ethyl 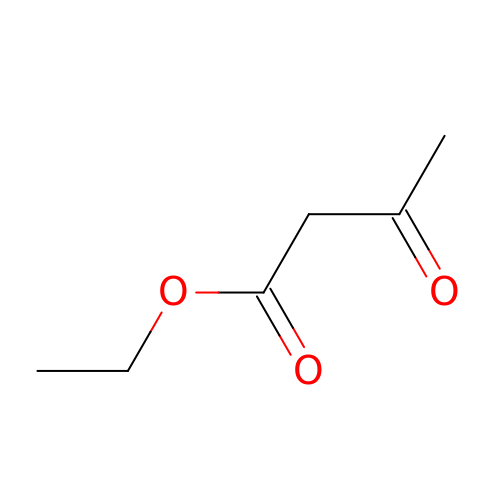3-oxobutanoate | C6 H10 O3 | XYIBRDXRRQCHLP-UHFFFAOYSA-N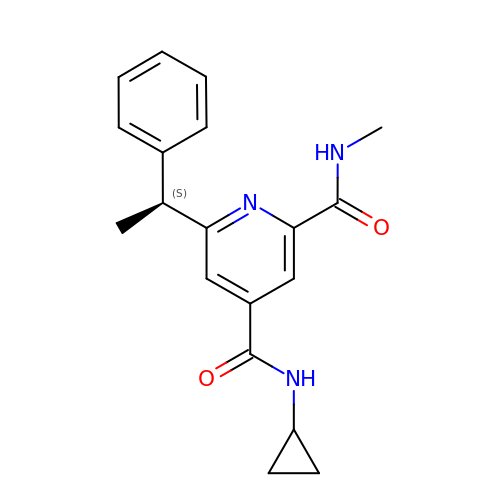~{N}4-cyclopropyl-~{N}2-methyl-6-[(1~{S})-1-phenylethyl]pyridine-2,4-dicarboxamide | C19 H21 N3 O2 | VGUKTEKHFHLCSV-LBPRGKRZSA-N>[2x]QNPYTELLVLKAHHDIVRFLVQLDDYRFASAGDDGIVVVWNAQTGEKLLELNGHTQKITAIITFPSLESCEEKNQLILTASADRTVIVWDGDTTRQVQRISCFQSTVKCLTVLQRLDVWLSGGNDLCVWNRKLDLLCKTSHLSDTGISALVEIPANCVV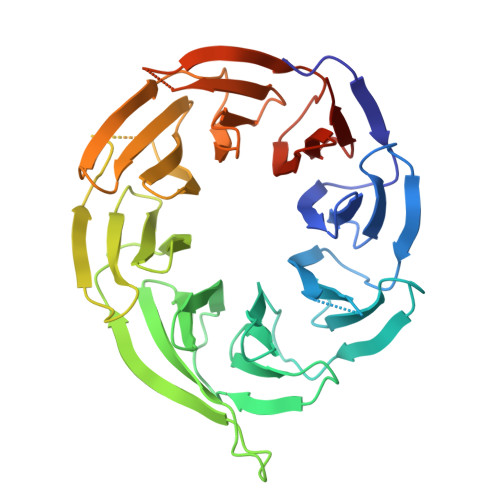AAVGKELIIFRLVAPTEGSLAWAILEVKRLLDHQDNILSLINVNDLSFVTGSHVGELIIWDALDWTMQAYERNFWDPSPQLDTQQEIKLCQKSNDISIHHFTCDEENVFAAVGRGLYVYSLQMKRVIACQKTAHDSNVLHVARLPNRQLISCSEDGSVRIWELREKQQLELIGDLIGHSSSVEMFLYFEDHGLVTCSADHLIILWKNGERESGL> SNAPGELKSVLRFKKLTEHAFTPSKGSKF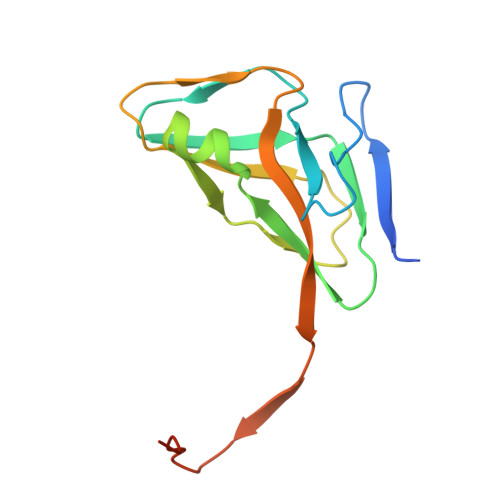AAGFDLCSAYDLVIPAVGKALVKTDIQVELPEGCYGRIAPRSGLSWKHHIDVGAGVIDRDYRGNVGVVLFNHAKTDYEVKKGDRVAQLICEKIIYPEIQEVEELMETERGEGGFGSTGNQ> GSHMASVDKKFLSGDPNIVDGQVDPGSAIPGDYAIEVVQLAQKPAAMSNGFPDKDQTQIGVGYIKFETPEGTKEVYINGSNSTLDGVMKQINAANVGLKAQVVEDRKDQENPFKLLVSGLSTGNDSQVTFPKIYLLDGDQDMYFEESRKAQNAKVKVDGFEIELPDNKSTDLVPGVTLDFKSAAPGREIRL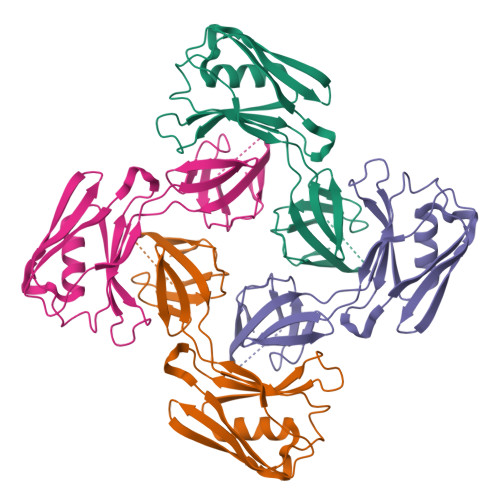SVKEN>[4x]MNHKVHMMSKPVLYYDDISPPVRGVLLTVAALGIKDQVELKLVRLFEREHLLEDFVKLNPLHAVPVLKHDDLVLTDSHAIIMYLCDIFGQDGDFSLKDPKQRARVHNRLCFNNAVLFQRESIVMRGLINRSIVTLEDHHLKPVQEAYDCLEVYLTNSKFVACDQLTVADFPIVACMSTVGMVCPLSTSRWPKTAAWFETMKQLPYYQQANQVGVDKLKERLHAVMKK

Here, we report that some flavonoids act as the inhibitors of the Ae. aegypti Noppera-bo (AeNobo) protein, which belongs to the glutathione S-transferase (GST) epsilon subfamily. Nobo plays a specialized role in the biosynthesis of the principal insect steroid hormones, ecdysteroids. As ecdysteroids are particularly important for the life cycle of insects, it is expected that a chemical inhibitor of ecdysteroidogenic enzymes, including Nobo, would be an insect growth regulator (IGR) that impacts insect development without affecting organisms other than insects. AeNobo adopts a canonical GST fold, which has a well-conserved GSH-binding site (G-site) and a hydrophobic substrate-binding pocket (H-site) adjacent to the G-site.

Next, crystal structures of AeNobo-GSH complexed with daidzein (AeNobo-GSH-daidzein) and luteolin (AeNobo-GSH-luteolin) were determined at 1.95 Å and 1.50 Å resolution, respectively. Daidzein and luteolin inhibited AeNobo enzymatic activity with an IC50 value of 3.87 μM and 3.99 μM, respectively; these compounds are known to exhibit larvicidal activity toward Ae. aegypti. Although daidzein and luteolin both bind to the AeNobo H-site, the binding orientations of daidzein and luteolin in the H-site are opposite to each other. The A-ring of daidzein is nested deep inside the H-site, but the A-ring of luteolin is located at the entrance of the H-site. The Oε of Glu-113 forms a hydrogen bond with the hydroxyl group at C7 of daidzein and two hydroxyl groups at C3′ and C4′ of luteolin. In the case of luteolin derivatives, apigenin, which lacks a hydroxyl group at C3′, exhibited a substantial decrease in its inhibitory activity having an IC50 value >25 μM. Moreover, chrysin, which lacks two hydroxyl groups at C3′ and C4′, did not exhibit any inhibitory activity. In contrast, 7,3′4′-trihydroxyflavone and 5,3′4′-trihydroxyflavone, both of which are luteolin derivatives but lack hydroxyl groups at C5 and C7, respectively, retained inhibitory activity against AeNobo to a level comparable to that of luteolin. These data suggest that the hydroxyl groups at C3′ and C4′ of luteolin are critical for the inhibition. As the hydroxyl residue at C7 of luteolin is close to Phe-39, the A-ring of luteolin cannot form a CH-π interaction with Phe-39.>[4x]HMSVNKVTCLVCRKGDNDEFLLLCDGCDRGCHIYCHRPKMEAVPEGDWF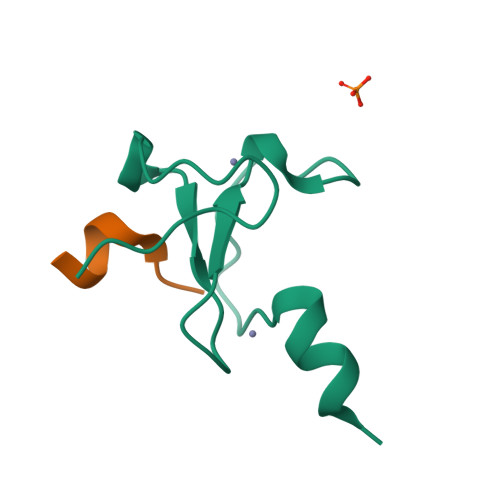CTVCLAQQV;>ARTKQTARKS[2x]> AAAAAAAAAAAAAAAAAAAAFKSTTQLIQQVSLTDFFRPDIEHAGSTVLILRHPTDLPALARHRAPPGRQTERLAEAWGQLLEASRAYVTSLSFIAACRAEEYTDKQAAEANRTAIVSAYGCSRMGARLIRFSECLRAMVQCHVFPHRFISFFGSLLEYTIQDNLCNITAVAKGPQEAARTDKTSTRRVTAN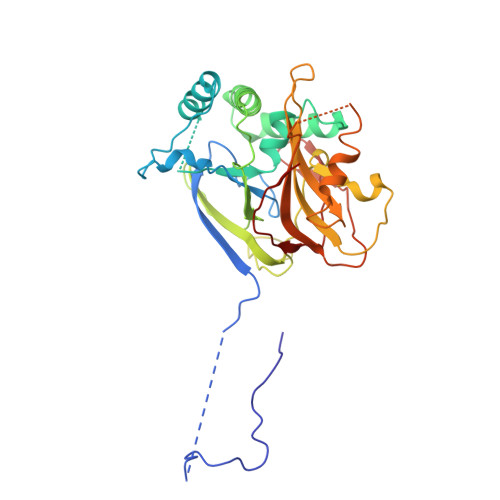IPACVFWDVDKDLHLSADGLKHVFLVFVYTQRRQREGVRLHLALSQLNEQCFGRGIGFLLGARICMYAAYTLIGTIPSESVRYTRRMERFGGYNVPTIWLEGVVWGGTNTWNEC[(2~{R})-2,3-bis(oxidanyl)propoxy]-[2-methyl-5-(trifluoromethyl)pyrazol-3-yl]borinic acid | C8 H12 B F3 N2 O4 | 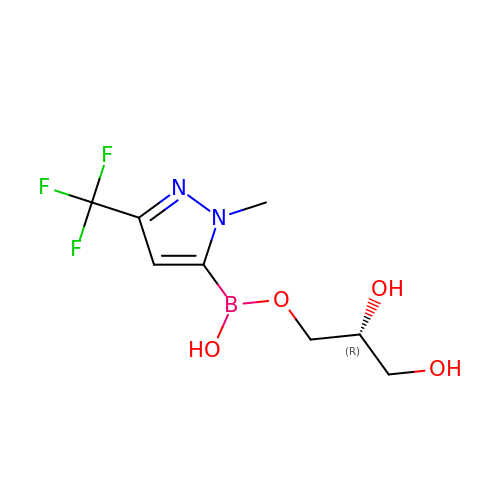YSSTVIJJFZPQNG-UHFFFAOYSA-N> XALYPYFLPIS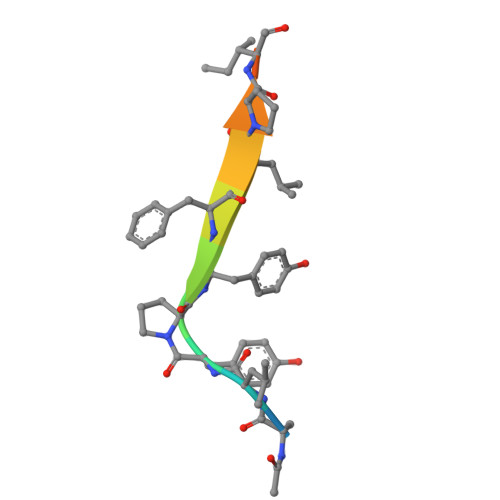AK>[2x]SNAMIPLFKVAVSPTALDRVAEVFASGYLGQGPRVAEFESALAARLGNPRVVSVHSGTSGLCLALRLLDAPEERDEVLSTPLTFEATNWAILADGRRITWVDVDPATLTMDLDDLERKISPATRAIIV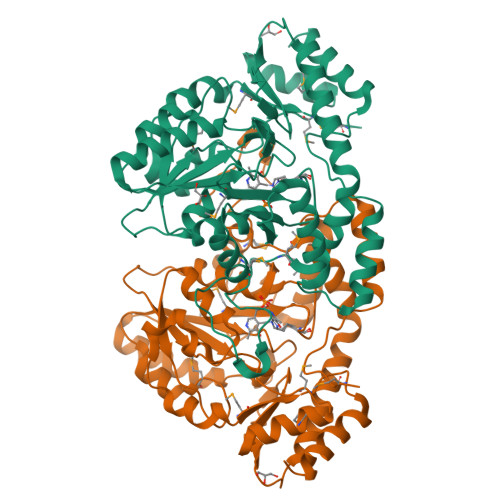VHWTGYPVDLDRLAGILDRAEREHGFRPAVIEDCAHAWGASYRGVPLGSHGNMCVFSFQALKHLTCGDGGLLTLPGDELHERAMLRRFYGIDRTADRLRGAYDVAEWGLKWHMTDLNAAIGLANLETVDEQLRLHRENAAFYDKELTGVPGLELLQRSPDREGSFYVYDVKVDDRPAFHRKMEAAGIMAGLVSRRNDEHSCVAHLRTSLPGLDSVYDRMVSLPVGWWLTEQDREHVVATIRSGW{[(1S)-2-(2-amino-6-oxo-1,6-dihydro-9H-purin-9-yl)-1-(hydroxymethyl)ethoxy]methyl}phosphonic acid | C9 H14 N5 O6 P | 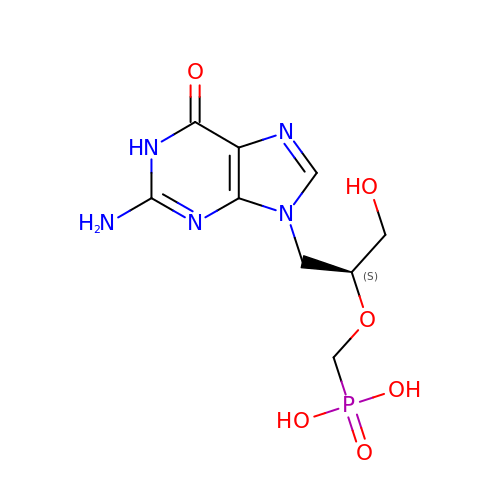VXDNQJCXIVLMQW-YFKPBYRVSA-N phenylmethanesulfonic acid | C7 H8 O3 S | 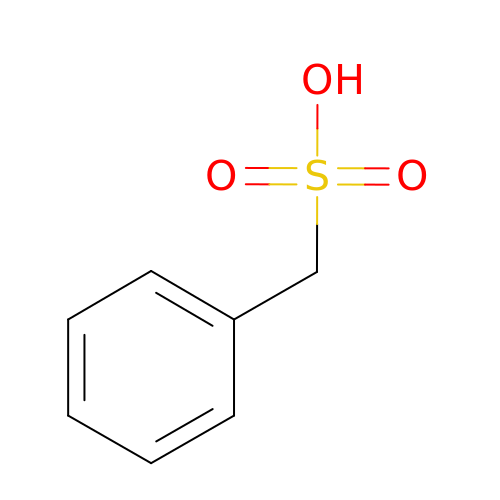NIXKBAZVOQAHGC-UHFFFAOYSA-N2-[4-(2-chloro-6-methylpyridin-3-yl)phenyl]-6-fluoro-3-methylquinoline-4-carboxylic 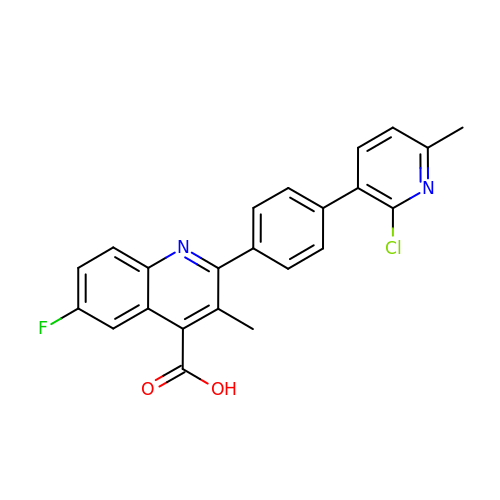acid | C23 H16 Cl F N2 O2 | NPMKPVGSRBWMIO-UHFFFAOYSA-N1-(1-{(2S)-1-[(3R,5R)-3,5-dimethylpiperazin-1-yl]-1-oxopropan-2-yl}piperidin-4-yl)-1,3-dihydro-2H-benzimidazol-2-one | C21 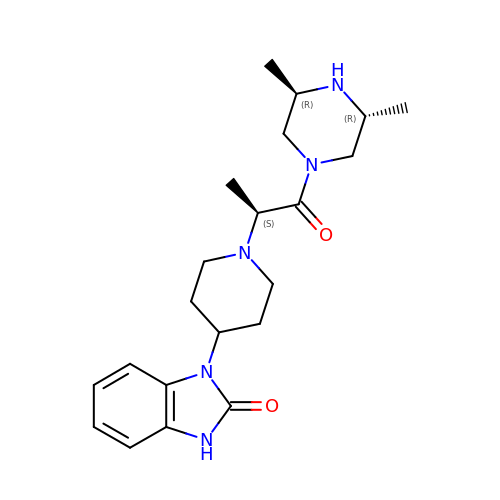H31 N5 O2 | LWPPVRZWNRKLJH-OAGGEKHMSA-N>[4x]MNVVSKTVSLPLKPREFGFFIDGEWRAGKDFFDRSSPAHDVPVTRIPRCTREDLDEAVAAARRAFENGSWAGLAAADRAAVLLKAAGLLRERRDDIAYWEVLENGKPISQAKGEIDHCIACFEMAAGAARMLHGDTFNNLGEGLFGMVLREPIGVVGLITPWNFPFMILCERAPFILASGCTLVVKPAEVTSATTLLLAEILADAGLPKGVFNVVTGTGRTVGQAMTEHQDIDMLSFTGSTG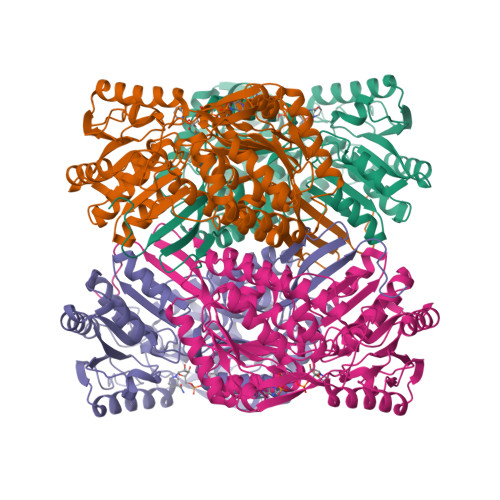VGKSCIHAAADSNLKKLGLELGGKNPIVVFADSNLEDAADAVAFGISFNTGQCCVSSSRLIVERSVAEKFERLVVAKMEKIRVGDPFDPETQIGAITTEAQNKTILDYIAKGKAEGAKLLCGGGIVDFGKGQYIQPTLFTDVKPSMGIARDEIFGPVLASFHFDTVDEAIAIANDTVYGLAASVWSKDIDKALAVTRRVRAGRFWVNTIMSGGPETPLGGFKQSGWGREAGLYGVEEYTQIKSVHIETGKRSHWISHHHHHH N-hydroxy-4-{[3-(2-hydroxyethyl)-1H-indol-1-yl]methyl}benzamide | C18 H18 N2 O3 | 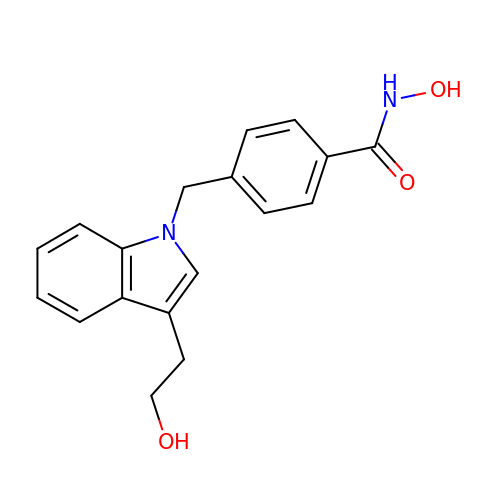ACXGELCLQKZFMQ-UHFFFAOYSA-N> GPGYQDPNSQIIPSMSVSIYPSSAEVLKACRNLGKNGLSNSSILLDKCPPPRPPSSPYPPLPKDKLNPPTPSIYLENKRDAFFPPLHQFCTNPNNPVTVIRGLAGALKLDLGLFSTKTLVEANNEHMVEVRTQLLQPADENWDPTGTKKIWHCESNRSHTTIAKYAQYQASSFQESLREENEKRSHHKDHSDSESTSSDNSGRRRKGPFKTIKFGTNIDLSDDKKWKLQLHELTKLPAFVRVVSAGNLLSHVGHTILGMNTVQLYMKVPGSRTPGHQENNNFCSVNINIGPGDC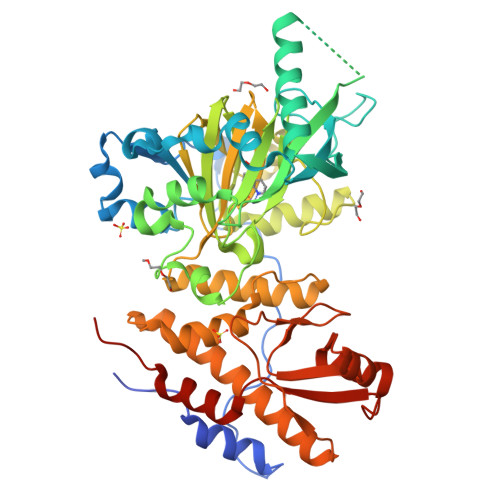EWFVVPEGYWGVLNDFCEKNNLNFLMGSWWPNLEDLYEANVPVYRFIQRPGDLVWINAGTVHWVQAIGWCNNIAWNVGPLTACQYKLAVERYEWNKLQSVKSIVPMVHLSWNMARNIKVSDPKLFEMIKYCLLRTLKQCQTLREALIAAGKEIIWHGRTKEEPAHYCSICEVEVFDLLFVTNESNSRKTYIVHCQDCARKTSGNLENFVVLEQYKMEDLMQVYDQFTLAPPLPSASS> AGDAAAGQAKAAVCGACHGADGNSPAPNFPKLAGQGERYLLKQMHDIKDGKRTVLEMTGLLTNLSDQDLADIAAYFASQKMSVGMADPNLVAQGEALFRGGKIAEGMPACTGCHSPSGVGIATAGFPHLGGQHATYVAKQLTDFREGTRTN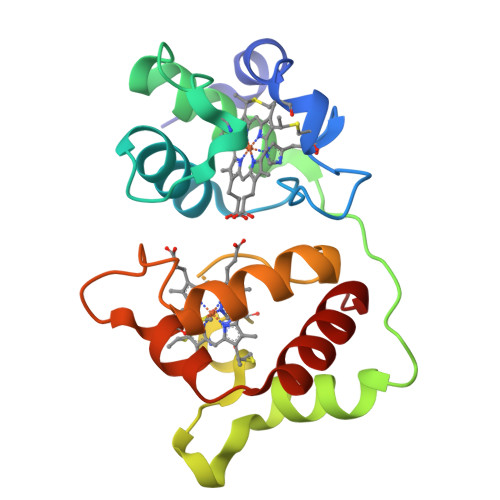DGDTKIMQSIAAKLSNKDIAAISSYIQGLH> EASATGTFIEQPNATECDFSPMLTGVAPQVYNFKRLVFSNCNYNLTKLLSLF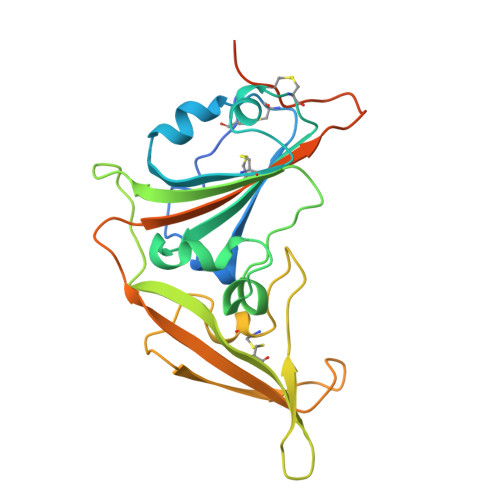AVDEFSCNGISPDSIARGCYSTLTVDYFAYPLSMKSYIRPGSAGNIPLYNYKQSFANPTCRVMASVLANVTITKPHAYGYISKCSRLTGANQDVETPLYINPGEYSICRDFSPGGFSEDGQVFKRTLTQFEGGGLLIGVGTRVPMTDNLQMSFIISVQYGTGTDSVCPMLDLGDSLTITNRLGKCVDYHHHHHH> MALDGIRMPDGCYADGTWELSVHVTDLNRDVTLRVTGEVHIGGVMLKLVEKLDVKKDWSDHALWWEKKRTWLLKTHWTLDKCGIQADAKLQFTPQHKLLRLQLPNMKYVKVKVNFSDRVFKAVSD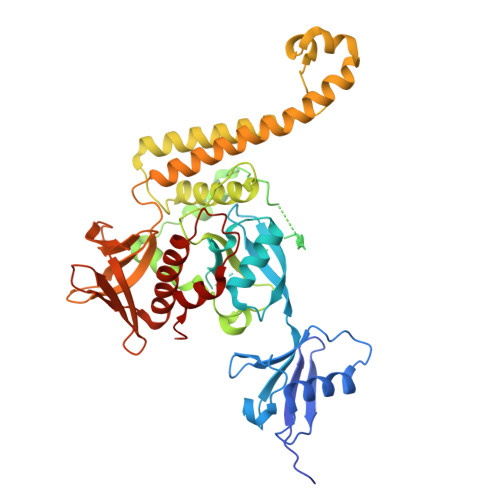ICKTFNIRHPEELSLLKKPRDPTKKKKKKLDDQSEDEALELEGPLIMPGSGSIYSSPGLYSKTMTPTYDAHDGSPLSPTSAWFGDSALSEGNPGILAVSQPVTSPEILAKMFKPQALLDKAKTNQGWLDSSRSLMEQDVKENEALLLRFKYYSFFDLNPKYDAIRINQLYEQAKWALLLEEIECTEEEMMMFAALQYHINKLSIMTSENHLTTDVNPECLVSPRYLKKYKSKQITARILEAHQNVAQMSLIEAKMRFIQAWQSLPEFGITHFIARFQGGKREELIGIAYNRLIRMDASTGDAIKTWRFSNMKQWNVNWEIKMVTVEFADEVRLSFICTEVDCKVVHEFIGGYIFLSTRAKDQNESLDEEMFYKLTSGWV>GSREEPSDLEELEQFAKTFKQRRIKLGFTQGDVGLAMGKLYGNDFSQTTISRFEALNLSFKNMCKLKPLLEKWLNDAENLSSDSSLSSPSALNSPGIEGLSRRRKKRTSIETNIRVALEKSFLENQKPTSEEITMIADQLNMEKEVIRVWFCNRRQKEKRINP[2x];>MLWQKPTAPE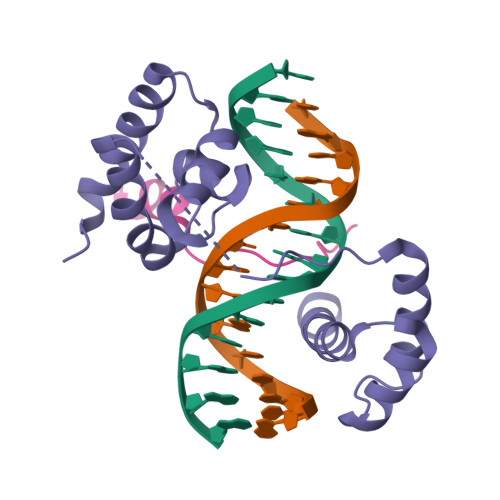QAPAPARPYQGVRVKEPVKELLRRKRGHASSGAA[2x]>MEHNYEDIAQEFIDFIYKNPTTYHVVSFFAELLDKHNFKYLSEKSNWQDSIGEDGGKFYTIRNGTNLSAFILGKNWRAEKGVGVIGSHVDALTVKLKPVSFKDTAEGYGRIAVAPYGGTLNELWLDRDLGIGGRLLYKKKGTNEIKSALVDSTPLPVCRIPSLAPHFGKPAEGPFDKEDQTIPVIGFPTPDEEGNEPPTDDEKKSPLFGKHCIHLLRYVAKLAGVEVSELIQMDLDLFDVQKGTIGGIGKHFLFAPRLDDRLCSFAAMIALICYAKDVNTEESDLFSTVTLYDNEEIGSLTRQGAKGGLLESVVERSSSAFTKKPVDLHTVWANSIILSADVNHLYNPNFPEVYLKNHFPVPNVGITLSLDPNGHMATDVVGTALVEELARRNGDKVQYFQIKNNSRSGGTIGPSLASQTGARTIDLGIAQLSMH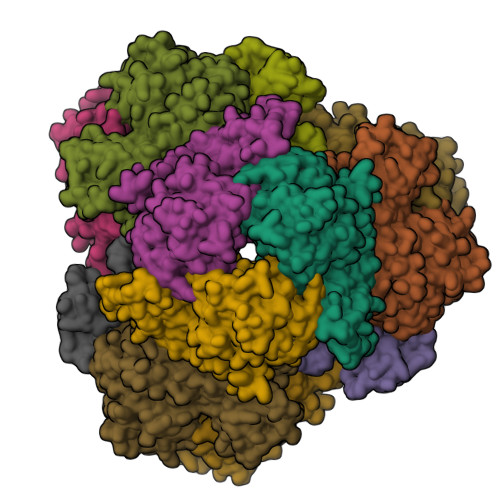SIRAATGSKDVGLGVKFFNGFFKHWRSVYDEFGEL[4x]> MGSSHHHHHHGSMMEFILSHVEKGVMTLTLNRPERLNSFNDEMHAQLAECLKQVERDDTIRCLLLTGAGRGFCAGQDLNDRNVDPTGPAPDLGMSVERFYNPLVRRLAKLPKPVICAVNGVAAGAGATLALGGDIVIAARSAKFVMAFSKLGLIPDCGGTWLLPRVAGRAR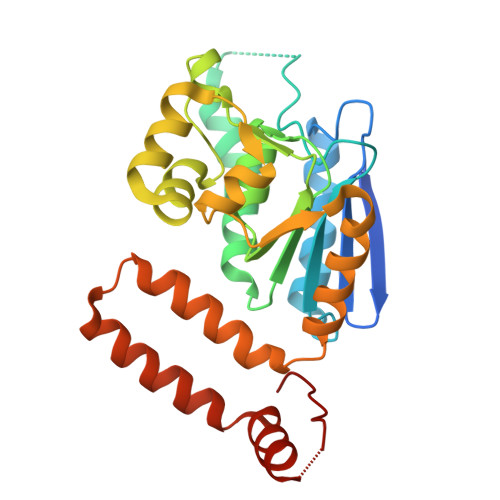AMGLALLGNQLSAEQAHEWGMIWQVVDDETLADTAQQLARHLATQPTFGLGLIKQAINSAETNTLDTQLDLERDYQRLAGRSADYREGVSAFLAKRSPQFTGK> DWVIPPINLPENSRGPFPQELVRIRSDRDKNLSLRYSVTGPGADQPPTGI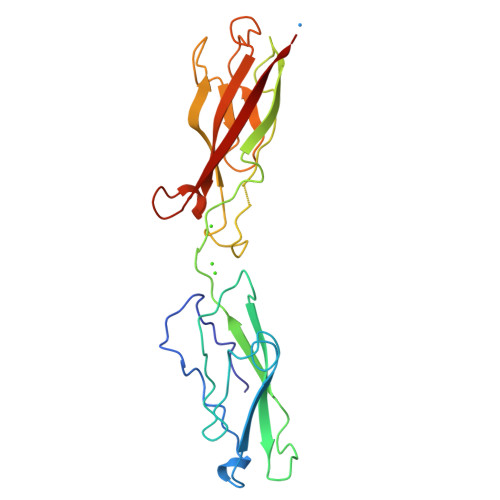FIINPISGQLSVTKPLDRELIARFHLRAHAVDINGNQVENPIDIVINVIDMNDNRPEFLHQVWNGSVPEGSKPGTYVMTVTAIDADDPNALNGMLRYRIVSQAPSTPSPNMFTINNETGDIITVAAGLDREKVQQYTLIIQATDMEGNPTYGLSNTATAVITVTD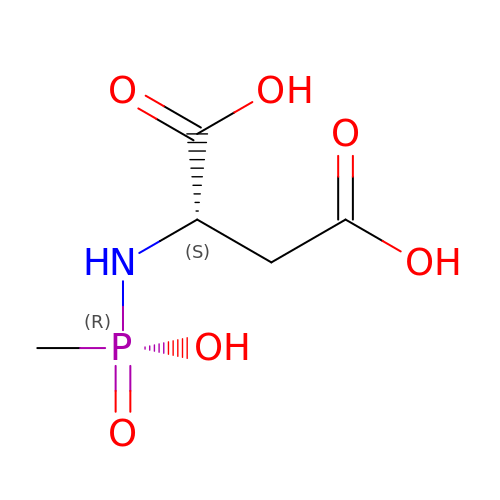N-[HYDROXY(METHYL)PHOSPHORYL]-L-ASPARTIC ACID | C5 H10 N O6 P | GKKRPYJQMIDFSC-VKHMYHEASA-N>[2x]GCGCGGAAACAAUGAUGAAUGGGUUUAAAUUGGGCA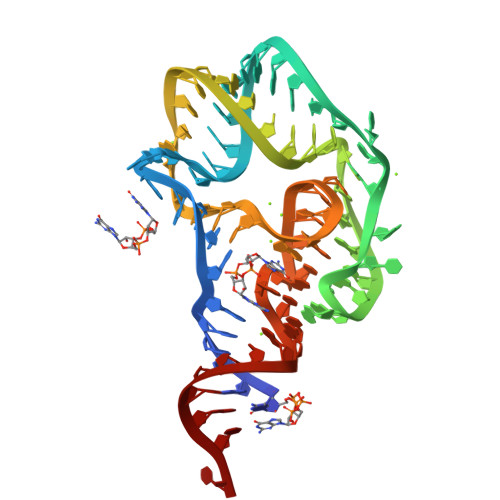CUUGACUCAUUUUGAGUUAGUAGUGCAACCGACCGUGCU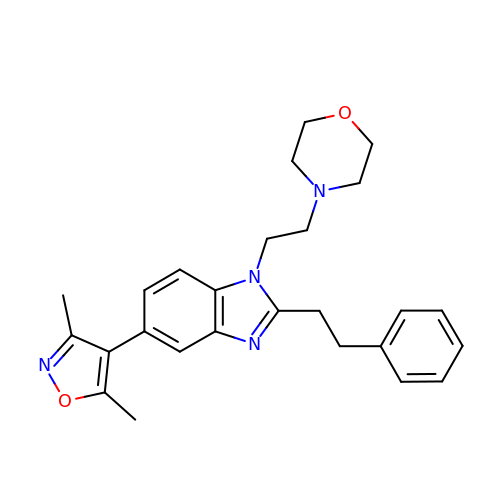5-(3,5-dimethyl-1,2-oxazol-4-yl)-1-[2-(morpholin-4-yl)ethyl]-2-(2-phenylethyl)-1H-benzimidazole | C26 H30 N4 O2 | ZVYCZICBBIUVHC-UHFFFAOYSA-N[(1S,2S,5R)-5-methyl-2-propan-2-yl-cyclohexyl]methanamine 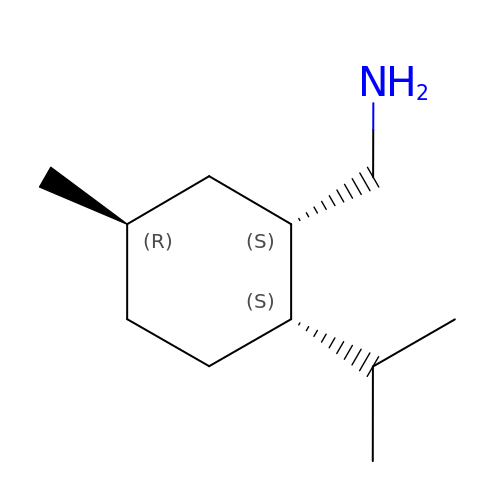| C11 H23 N | BMNCNNYYLCTHDB-MXWKQRLJSA-N>AMKHGIYYAYWEQEWEADYKYYIEKVAKLGFDILEIAA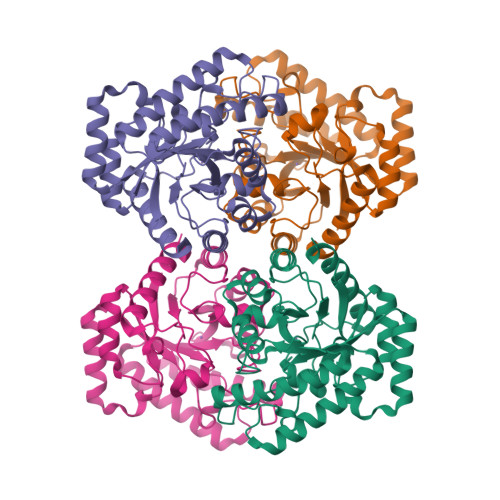SPLPFYSDIQINELKACAHGNGITLTVGHGPSAEQNLSSPDPDIRKNAKAFYTDLLKRLYKLDVHLIGGALYSYWPIDYTKTIDKKGDWERSVESVREVAKVAEACGVDFCLEVLNRFENYLINTAQEGVDFVKQVDHNNVKVMLDTFHMNIEEDSIGGAIRTAGSYLGHLHTGECNRKVPGRGRIPWVEIGEALADIGYNGSVVMEPFVRMGGTVGSNIKVWRDISNGADEKMLDREAQAALDFSRYVLECHKHS[4x]>GSEDFTFDGTKRLSVNYVKGILQPTDTCDIWDKIWNFQAKPDDLLISTYPKAGTTWTQEIVELIQNEGDVEKSKRAPTHQRFPFLEMKIPSLGSGLEQAHAMPSPRILKTHLPFHLLPPSLLEKNCKIIYVARNPKDNMVSYYHFQRMNKALPAPGTWEEYFETFLAGKVCWGSWHEHVKGWWEAKDKHRILYLFYEDMKKNPKHEIQKLAEFIGKKLDDKVLDKIVHYTSFDVMKQNPMANYSSIPAEIMDHSISPFMRKGAVGDWK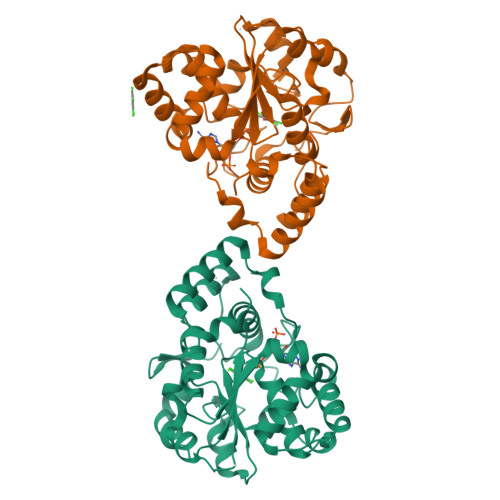KHFTVAQNERFDEDYKKKMTDTRLTFHFQF[2x]pmcThe CCAAT/enhancer-binding protein (C/EBP) transcription factors belong to the basic region-leucine zipper (bZIP) family of transcription factors, which play crucial roles in tissue development, cell proliferation, and differentiation. In humans, ten C/EBP transcription factors have been identified, including six C/EBP proteins (named C/EBPα-ζ), and four C/EBP-related proteins, TEF, HLF, DBP, and NFIL3 (8, 9, 10, 11). The bZIP domain consists of a basic region (BR) and a leucine zipper region with a sequence of heptad repeats. The leucine zipper region is responsible for the dimerization of the bZIP domain, allowing the bZIP proteins to form either homodimers or heterodimers.

Our ITC results showed that C/EBPα and C/EBPβ bound to the TTACGTAA DNA with a Kd of ∼0.354 μM and 0.018 μM, respectively, which were 1.4- or 3.8-fold stronger than to the TTGCGCAA DNA, i.e., the reported consensus binding sequence of C/EBPα/β. To understand why C/EBPα/β prefers recognizing the TTACGTAA DNA, we determined the structures of C/EBPα and C/EBPβ in complex with the TTACGTAA DNA, respectively. Our ITC results showed that the binding affinity of NFIL3 to the TTACGTAA DNA was ∼ 2-fold weaker than that of C/EBPβ. Sequence analysis of the DNA binding basic region showed that the A87 in NFIL3 was substituted by V285 in C/EBPβ. By comparing the structures of the NFIL3-TTACGTAA complex and the C/EBPβ-TTACGTAA complex, we found that the longer side chain of V285 in C/EBPβ could form extra van der Waals interactions and an O•••H-C hydrogen bond with T4 on the T4/A4' base pair compared to A87 of NFIL3. The longer side chain of V285 could also form van der Waals interactions with R289 to attract the latter to form bidentate hydrogen bonds with G6' in the C6/G6' base pair. Structural comparison showed that the shorter side chain of D320 in C/EBPα prevented it from forming additional hydrogen bonds with N321' in the other monomer, unlike E111 in NFIL3 or E309 in C/EBPβ that formed a hydrogen bond with N112' in NFIL3 or N321' in C/EBPβ from the other monomer. On the other hand, mutating E111 of NFIL3 or E309 of C/EBPβ to D resulted in ∼8- or 4-fold weaker binding affinities than their wild-type counterparts, respectively.

>[2x]GVKSKAKKTVDKHSDEYKIRRERNNIAVRKSRDKAKMRNLETQHKVLELTAENERLQKKVEQLSRELSTLRNLFKQLPE>UAAGUUCUCGAUCUUUAAAAUCGUUAGCUCGCCAGUUAGCGAGGUCUGCGAAAGCAGAUAAUCGGGUGCAACUCCCGCCCUUUCUCCGAGGGUCAUCGGAACCA[2x]

The 3′-UTR of the species turnip yellow mosaic virus (TYMV) is an important model for exploring important principles of RNA structure-based translational control. The 3′-most domain of the TMYV 3′-UTR is the transfer RNA (tRNA)-like structure (TLS) that mimics tRNA to drive aminoacylation (with valine) of the viral RNAs. However, deletion or mutation of the UPD decreases TLS-dependent aminoacylation and the presence of the UPD stabilizes the overall fold of the TLS, implying the existence of interdomain structural and functional coupling. Specifically, the UPD acts as a structure-based ribosome sensor, communicating its conformational status to the TLS to alter the efficiency of downstream functions.

Therefore, we solved the structure of the entire TYMV 3′-UTR by x-ray crystallography to a resolution of 3.1 Å. The crystallographic asymmetric unit contains two copies of the RNA that are structurally almost identical; in both, all nucleotides except the 5′-terminal U and 3′-terminal CCA sequences had density of high enough quality that they could be built. The UPD forms a compact H-type pseudoknot. Consistent with this type of pseudoknot, Loop 1 (L1, nucleotides 5–7) lies in the major groove of Stem 2 (S2), with U5 and U6 pairing with the Hoogsteen edges of A19 and A20, respectively (the latter forms a base triple). In addition, a previously unpredicted non-canonical base pair forms between U8 and U24; this pair stacks on Stem 2. Surprisingly, the UPD assumes an angle roughly perpendicular to the TLS’ helices with no direct contact between the two domains. First, there are two RNA molecules in the asymmetric unit with different crystal contacts but identical UPD positions; this is highly unlikely to occur if crystal packing dictates the interdomain orientation. Although nucleotides in the linker are not base paired, they form a well-defined structure containing several unusual features. The linker structure appears to be stabilized by extensive base stacking: the non-canonical U8:U24 base pair (not previously predicted) in the UPD stacks with U25; A26 stacks directly between U25 and the syn-G27:C94 base pair (within the Z-DNA-like element). The high-resolution structure reveals that the linker is part of a “spine” of continuously stacked nucleobases that extends from the UPD, through the linker, to the TLS’ V-region and the D-loop at A38, which interacts with the T-loop.>GSMPLLLDDGDPKAQTGFDLSTATTLFWRPVPVHVKQQDREDVLEELTFRILTGVAKQNHNLRILRIHISSDSDLFFLHTLEVSEEDFQSLKNDEDILVDFASFPGKIISLLEKCILAQPGDSPRFQAVLTIRGGESVFK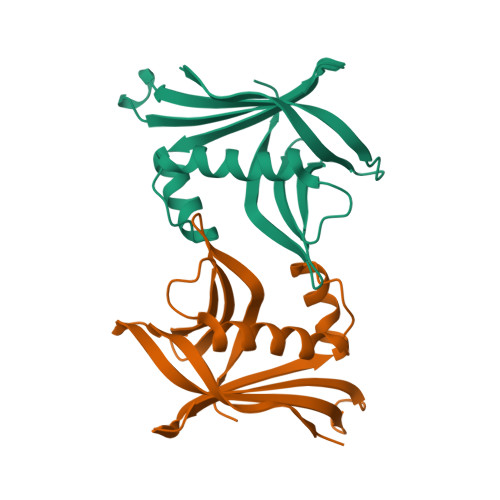IVEINDFRRLPHITLAFRPGN[4x]>[4x]MVTLSGRIPLGGQVTDLGYAAGWRLVRA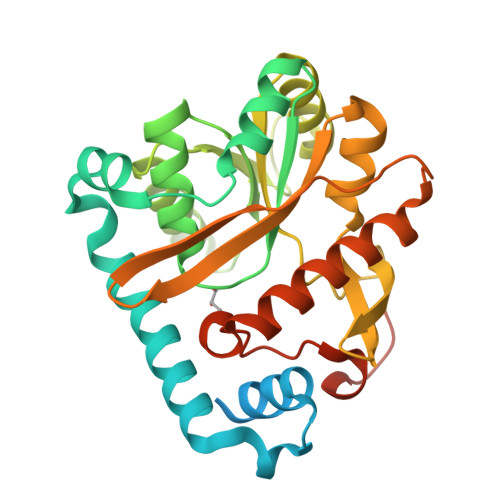MPEAMAQGVFGAGARYAARNGGPEQLRRNLARVVGKPPADVPDDLIRASLASYARYWREAFRLPAMDHGRLGEQLDVIDIDHLWSALDAGRGAVLALPHSGNWDMAGVWLVQNYGPFTTVAERLKPESLYRRFVEYRESLGFEVLPLTGGERPPFEVLAERLTDNRPICLMAERDLTRSGVQVDFFGEATRMPAGPAKLAIETGAALFPVHCWFEGDGWGMRVYPELDTSSGDVTAITQALADRFAANIATYPADWHMLQPQWIADLSDERRARLGTSRHHHHHH>[2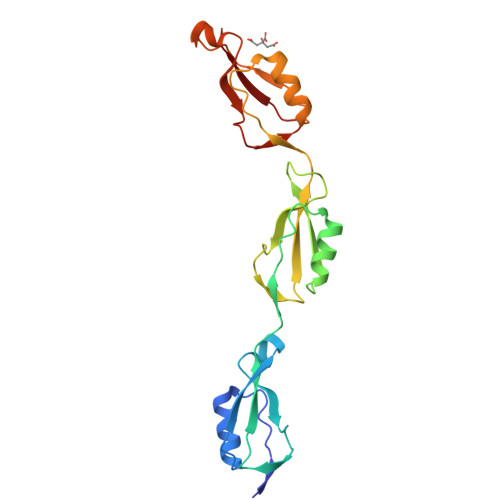x]GPEQREIPDVSTLTYAEAVKKLTAAGFGRFKQANSPSTPELVGKVIGTNPPANQTSAITNVVIIIVGSGPATKDIPDVAGQTVDVAQKNLNVYGFTKFSQASVDSPRPAGEVTGTNPPAGTTVPVDSVIELQVSKGNQFVMPDLSGMFWVDAEPRLRALGWTGMLDKGADVDAGGSQHNRVVYQNPPAGTGVNRDGIITLRFGQ> GDERFYAEHLMPTLQGLLDPESAHRLAVRFTSLGLLPRARFQDSDMLEVRVLGHKFRNPVGIAAGFDKHGEAVDGLYKMGFGFVEIGSVTPKPQEGNPRPRVFRLPEDQAVINRYGFNSHGLSVVEHRLRARQQKQAKLTEDGLPLGVNLGKNKTSVDAAEDYAEGVRVLGPLADYLVVNVSSPNTAGLRSLQGKAELRRLLTKVLQERDGLRRVHRPAVLVKIAPDLTSQDKEDIASVVKELGIDGLIVTNTTVSRPAGLQGAL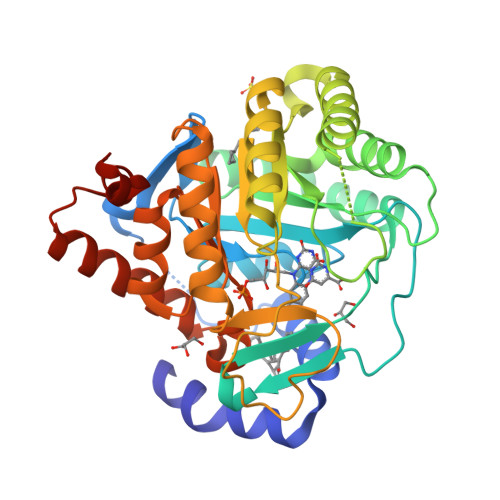RSETGGLSGKPLRDLSTQTIREMYALTQGRVPIIGVGGVSSGQDALEKIRAGASLVQLYTALTFWGPPVVGKVKRELEALLKEQGFGGVTDAIGADHRRLEHHHHHH>[4x]GSTIQ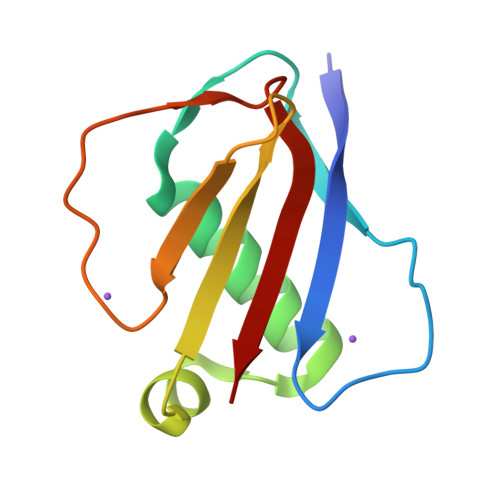IPYTITVNGTSQNILSSLTFNKNQNISYKDIENKVKSVLYFNRGISDIDLRLSKQAEYTVHFKNGTKRVIDLKSGIYTADLINTSDIKAISVNVD CYCLOPENTANAMINE | C5 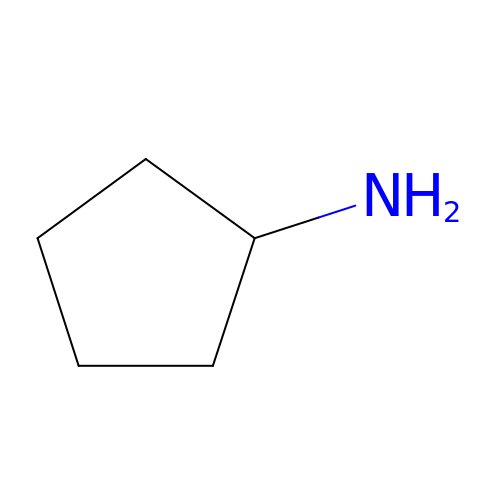H11 N | NISGSNTVMOOSJQ-UHFFFAOYSA-N> STSAGPTVPDRDNDGIPDSLEVEGYTVDVKNKRTFLSPWISNIHEKKGLTKYKSSPEKWSTASDPYSDFEKVTGRIDKNVSPEARHPLVAAYPIVHVDMENIILSKNEDQSTQNTDSQTRTISKNTSTSRTHTSEPGSNSNSSTVAIDHSLSLAGERTWAETMGLNTADTARLNANIRYVNTGTAPIY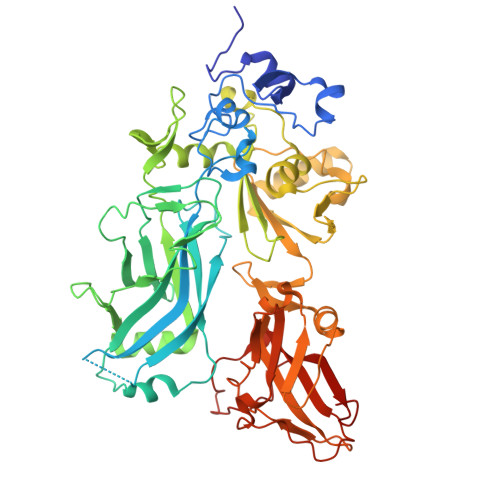NVLPTTSLVLGKNQTLATIKAKENQLSQILAPNNYYPSKNLAPIALNAQDDFSSTPITMNYNQFLELEKTKQLRLDTDQVYGNIATYNFENGRVRVDTGSNWSEVLPQIQETTARIIFNGKDLNLVERRIAAVNPSDPLETTKPDMTLKEALKIAFGFNEPNGNLQYQGKDITEFDFNFDQQTSQNIKNQLAELNATNIYTVLDKIKLNAKMNILIRDKRFHYDRNNIAVGADESVVKEAHREVINSSTEGLLLNIDKDIRKILSGYIVEIEDTEGLKEVINDRYDMLNISSLRQDGKTFIDFKKYNDKLPLYISNPNYKVNVYAVTKENTIINPSENGDTSTNGIKKILIFSKKGYEIG> ENLKLGFLVKQPEEPWFQTEWKFADKAGKDLGFEVIKIAVPDGEKTLNAIDSLAASGAKGFVICTPDPKLGSAIVAKARGYDMKVIAVDDQFV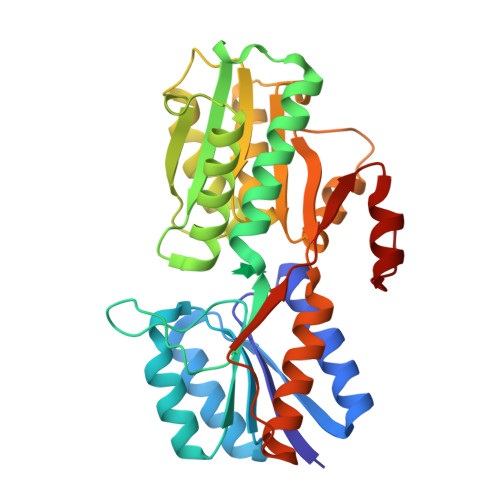NAKGKPMDTVPLVMMAATKIGERQGQELYKEMQKRGWDVKESAVMAITANELDTARRRTTGSMDALKAAGFPEKQIYQVPTKSNDIPGAFDAANSMLVQHPEVKHWLIVGMNDSTVLGGVRATEGQGFKAADIIGIGINGVDAVSELSKAQATGFYGSLLPSPDVHGYKSSEMLYNWVAKDVEPPKFTEVTDVVLITRDNFKEELEKKGLGGK> GSSAVNQENERLMEEYERLASELLEWIRRTIPWLENRTPEKTMQAMQKKLEDFRDYRRKHKPPKVQEKCQLEINFNTLQTKLRISNRPAFMPSEGKMVSDIAGAWQRLEQAEKGYEEWLLNEIRRLERLEHLAEKFRQKASTHETWAYGKEQILLQKDYESASLTEVRALLRKHEAFESDLAAHQDRVEQIAAIAQELNELDYHDAVNVNDRCQKICDQWDRLGTLTQKRREALERMEKLLETIDQLHLEFAKRAAPFNNWMEGAMEDLQDMFIVHSIEEIQSLITAHEQFKATLPEADGERQSIMAIQNEVEKVIQSYNIRISSSNPYSTVTMDELRTKWDKVKQLVPIRDQSLQEELARQHANERLRRQFAAQANAIGPWIQN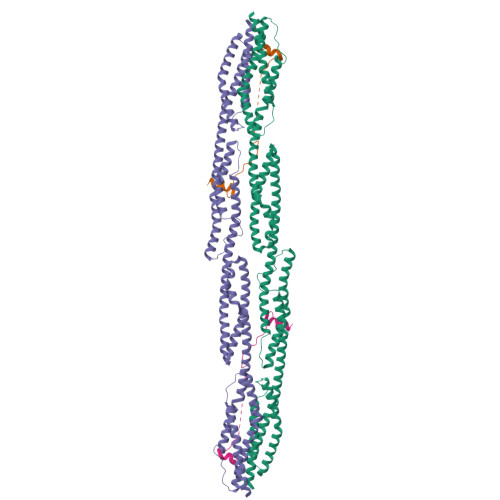KMEEIARSSIQITGALEDQMNQLKQYEHNIINYKNNIDKLEGDHQLIQEALVFDNKHTNYTMEHIRVGWELLLTTIARTINEVETQILTRD;> GPAMKHITVFKTYISPWERAMGVDPQQKMELGIDLLAYGAKAELPKYKSFNRTAMPYGGYEKASKRMTFQMPKFDLGPLLSEPLVLYNQNLS> MDKNRVFGQRLRQSIQNYFSSPWLLYTAKAEALLDLRDDEAMLNEMEAVGELPMALEYESLTDV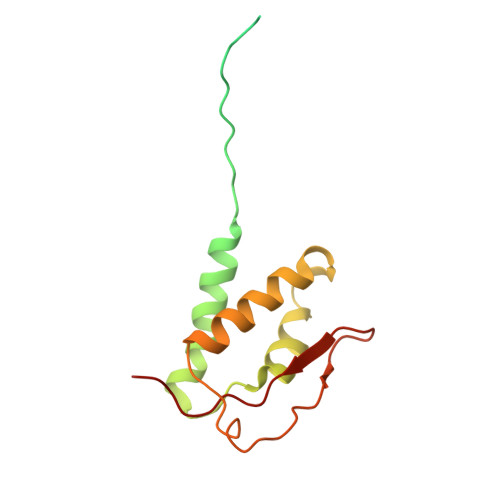QTQIVTAIQAELAHFRNTAQPINLGAVLQEQLARYPQSRHFDVARIIVDQAVKLGMASQDHQAVYPVWQPIDDFSAAVQAHLIDQYDK> MGSDKIHHHHHHMITDENKKLAQWAMDYALKNGCQAAKVLLYSSSNTSFELRDAKMDRLQQASEGGLSLSLYVDGRYGSISTNRLNRKELETFIKNGIDSTRYLAKDEARVLADPSRYYKGGKPDLKLYDAKFASLNPDDKIEMAKAVAEEALGKDERIISVGSSYGDGEDFAYRLISNGFEGETKSTWYSLSADITIRGEGEARPSAYWYESSLYMNDLIKKGIGQKALERVLRKLGQKKVQSGKYTMVVDPMNSSRLLSPMISALNGSALQQKNSFLLNKLNEKI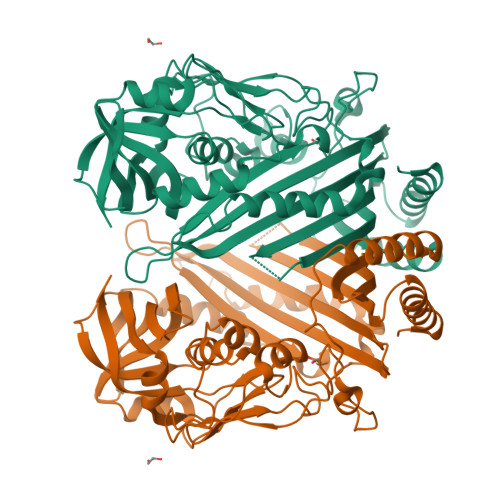ASDRLTLTDEPHLVKASGARYFDNEGIATERRSIFDKGVLNTYFIDTYNAKKMGVDPTISGSSILVMETGDKNLDGLIAGVEKGILVTGFNGGNNNSSTGDFSYGIEGFLIENGKLTQPVSEMNVTGNLITLWNSLVATGNDPRLNSSWRIPSLVFEGVDFSGL Mmi1 is an essential RNA-binding protein in the fission yeast Schizosaccharomyces pombe that eliminates meiotic transcripts during normal vegetative growth. A C-terminal YTH RNA-binding domain in Mmi1 recognizes UNAAAC motifs (where N is any ribonucleotide) that are present in multiple copies within DSRs. Surprisingly, Mmi1 binds DSR RNA using a divergent mechanism on a surface that is distinct from the m6A-binding pocket, including extended protein sequences located upstream and downstream of the YTH domain. We propose that the low-complexity region influences RNA binding indirectly by reducing dynamic motions of the RNA-binding groove and stabilizing a conformation of the YTH domain that binds to RNA with high affinity.

We were not successful in crystallizing the USR–YTH construct itself, but removal of an additional 19 residues from the N terminus allowed us to crystallize Mmi1 residues 301–488 bound to a 7-mer DSR RNA (UUAAACC). We determined its X-ray crystal structure to 1.4 Å resolution and built an atomic model for residues 315–488 and all seven nucleotides. The core YTH domain of our structure of Mmi1-RNA is similar to apo-Mmi1 and to previously reported structures with a central five-stranded β-sheet surrounded by four α-helices. Part of the N-terminal USR region of the polypeptide, which was line broadened in NMR spectra (making structural analysis of this region impossible by NMR), was ordered in the crystal structure and folds back to contact the back of the YTH domain. This results in a network of hydrophobic interactions involving residues Leu-316, Phe-318, and His-324 of the USR, Met-334 and Ile-335 from the N-clamp, and Met-465 and Arg-471 from the YTH domain. In summary, our structure shows that part of the low-complexity USR of Mmi1 (residues 315–326) lacks secondary structure elements but adopts a defined fold on RNA binding, forming contacts with the YTH domain. DSR RNA was bound in a pseudo-helical conformation in a groove generated by the central β-sheet and the C-terminal α-helix using both positively-charged and hydrophobic surfaces. Residues N- and C-terminal to the annotated YTH domain contact the 3′ and 5′ ends of the UNAAAC motif, respectively. Examination of relative B-factors from our crystal structures suggests that the final C-terminal helix is relatively rigid when bound to RNA. Residues 301–311 of the USR are not visible in our crystal structure, and signals from most of this region are line broadened in NMR experiments.

> SASRKEKPKARASTPPPLNFSRASEHRNEKGERISMINPRVVLDENGISHRSRYFIMLCDNETAIAHAKKTSIWAVKKDSSKRISDAYKKASVYFIFVAQQTYNALGYAQVVSDLNSTELPFWSDSSHAGGVRIKWIKTCNLFSAEISEIVSHMDHGSEARDGMEMMYDEGSRLCTLINYAIMKRIGRDR>[2x]GSHMELTPDQQTLLHFIMDSYNKQRMPQEITNKILKEAFSAEENFLILTEMATNHVQVLVEFTKKLPGFQTLDHEDQIALLKGSAVEAMFLRSAEIFNKKLPSGHSDLLEARIRNSGISDEYITPMFSFYKSIGELKMTQEEYALLTAIVILSPDRQYIKDREAVEKLQEPLLDVLQKLCKIHQPENPQHF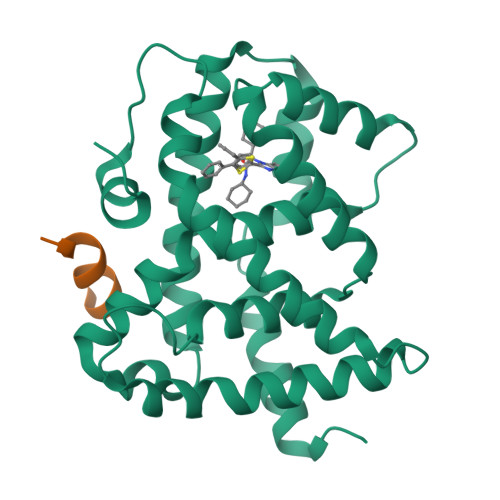ACLLGRLTELRTFNHHHAEMLMSWRVNDHKFTPLLCEIWDVQ;>[2x]KDHQLLRYLLDKDE> APSASFERRQGSVNPY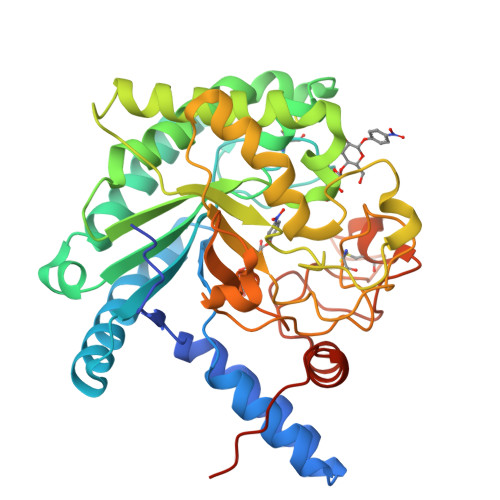IGRSPLVIKSYAEKLEETIAYFEAQGDELNAARTRTVQGIPTFAWISDSATIDTIQPLIADAVAHQEASGEQVLVQLVIYNLPDRDCAAKASDGEFHLDDDGANKYRAYVDRIVAELSTADADKLHFSIVLEPDSLGNMVTNMHVPKCQGAATAYKEGIAYTIASLQKPNIDLYIDAAHGGWLGWNDNLRPSAEIFKETLDLARQITPNATVRGLAINVSNYNPYKTRAREDYTEWNNAYDEWNYVKTLTPHLQAVGFPAQFIVDQGRSGREGIRTEWGQWCNIRNAGFGIRPTTDQAIVDSANVDAIVWVKPGGESDGTSDVNAVRFDENCRSPASHVPAPEAGEWFNEFVVNLVINANPPLEPTYAAAALEHHHHHH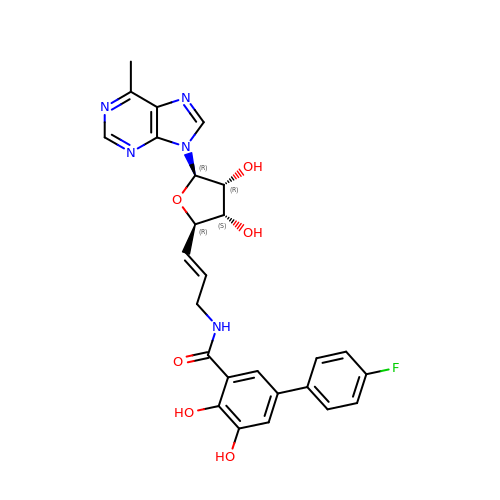N-[(E)-3-[(2R,3S,4R,5R)-3,4-dihydroxy-5-(6-methylpurin-9-yl)oxolan-2-yl]prop-2-enyl]-5-(4-fluorophenyl)-2,3-dihydroxy-benzamide | C26 H24 F N5 O6 | HPSAAEAALHAMSZ-ORAYEHMWSA-N>MNTQKPFENHLKSVDDLKTTYEEYRAGFIAFALEKNKRSTPYIERARALKVAASVAKTPKDLLYLEDIQDALLYASGISDKAKKFLTEDDKKESINNLIENFLEPAGEEFIDELIFRYLLFQGDSLGGTMRNIAGALAQQKLTRAIISALDIANIPYKWLDSRDKKYTNWMDKPEDDYELETFAKGISWTINGKHRTLMYNITVSLVKKNVDICLFNCEPEIYTPQKVHQQPEKYLLLGELKGGIDPAGADEHWKTANTALTRIRNKFSEKGLSPKTIFIGAAIEHSMAEEIWD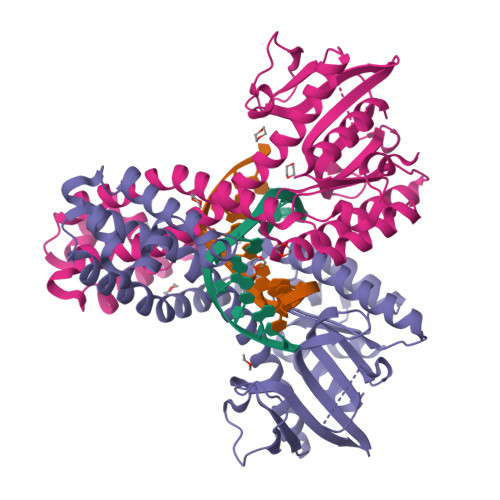QLQSGSLTNSANLTKTEQVGSLCRWIINI[2x]> MAFVATQGATVVDQ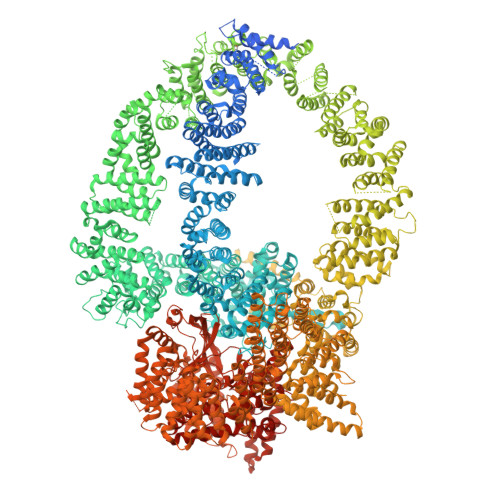TTLMKKYLQFVAALTDVNTPDETKLKMMQEVSENFENVTSSPQYSTFLEHIIPRFLTFLQDGEVQFLQEKPAQQLRKLVLEIIHRIPTNEHLRPHTKNVLSVMFRFLETENEENVLICLRIIIELHKQFRPPITQEIHHFLDFVKQIYKELPKVVNRYFENPQVIPENTVPPPEMVGMITTIAVKVNPEREDSETRTHSIIPRGSLSLKVLAELPIIVVLMYQLYKLNIHNVVAEFVPLIMNTIAIQVSAQARQHKLYNKELYADFIAAQIKTLSFLAYIIRIYQELVTKYSQQMVKGMLQLLSNCPAETAHLRKELLIAAKHILTTELRNQFIPCMDKLFDESILIGSGYTARETLRPLAYSTLADLVHHVRQHLPLSDLSLAVQLFAKNIDDESLPSSIQTMSCKLLLNLVDCIRSKSEQESGNGRDVLMRMLEVFVLKFHTIARYQLSAIFKKCKPQSELGAVEAALPGVPTAPAAPGPAPSPAPVPAPPPPPPPPPPATPVTPAPVPPFEKQGEKDKEDKQTFQVTDCRSLVKTLVCGVKTITWGITSCKAPGEAQFIPNKQLQPKETQIYIKLVKYAMQALDIYQVQIAGNGQTYIRVANCQTVRMKEEKEVLEHFAGVFTMMNPLTFKEIFQTTVPYMVERISKNYALQIVANSFLANPTTSALFATILVEYLLDRLPEMGSNVELSNLYLKLFKLVFGSVSLFAAENEQMLKPHLHKIVNSSMELAQTAKEPYNYFLLLRALFRSIGGGSHDLLYQEFLPLLPNLLQGLNMLQSGLHKQHMKDLFVELCLTVPVRLSSLLPYLPMLMDPLVSALNGSQTLVSQGLRTLELCVDNLQPDFLYDHIQPVRAELMQALWRTLRNPADSISHVAYRVLGKFGGSNRKMLKESQKLHYVVTEVQGPSITVEFSDCKASLQLPMEKAIETALDCLKSANTEPYYRRQAWEVIKCFLVAMMSLEDNKHALYQLLAHPNFTEKTIPNVIISHRYKAQDTPARKTFEQALTGAFMSAVIKDLRPSALPFVASLIRHYTMVAVAQQCGPFLLPCYQVGSQPSTAMFHSEENGSKGMDPLVLIDAIAICMAYEEKELCKIGEVALAVIFDVASIILGSKERACQLPLFSYIVERLCACCYEQAWYAKLGGVVSIKFLMERLPLTWVLQNQQTFLKALLFVMMDLTGEVSNGAVAMAKTTLEQLLMRCATPLKDEERAEEIVAAQEKSFHHVTHDLVREVTSPNSTVRKQAMHSLQVLAQVTGKSVTVIMEPHKEVLQDMVPPKKHLLRHQPANAQIGLMEGNTFCTTLQPRLFTMDLNVVEHKVFYTELLNLCEAEDSALTKLPCYKSLPSLVPLRIAALNALAACNYLPQSREKIIAALFKALNSTNSELQEAGEACMRKFLEGATIEVDQIHTHMRPLLMMLGDYRSLTLNVVNRLTSVTRLFPNSFNDKFCDQMMQHLRKWMEVVVITHKGGQRSDGNESISECGRCPLSPFCQFEEMKICSAIINLFHLIPAAPQTLVKPLLEVVMKTERAMLIEAGSPFREPLIKFLTRHPSQTVELFMMEATLNDPQWSRMFMSFLKHKDARPLRDVLAANPNRFITLLLPGGAQTAVRPGSPSTSTMRLDLQFQAIKIISIIVKNDDSWLASQHSLVSQLRRVWVSENFQERHRKENMAATNWKEPKLLAYCLLNYCKRNYGDIELLFQLLRAFTGRFLCNMTFLKEYMEEEIPKNYSIAQKRALFFRFVDFNDPNFGDELKAKVLQHILNPAFLYSFEKGEGEQLLGPPNPEGDNPESITSVFITKVLDPEKQADMLDSLRIYLLQYATLLVEHAPHHIHDNNKNRNSKLRRLMTFAWPCLLSKACVDPACKYSGHLLLAHIIAKFAIHKKIVLQVFHSLLKAHAMEARAIVRQAMAILTPAVPARMEDGHQMLTHWTRKIIVEEGHTVPQLVHILHLIVQHFKVYYPVRHHLVQHMVSAMQRLGFTPSVTIEQRRLAVDLSEVVIKWELQRIKDQQPDSDMDPNSSGEGVNSVSSSIKRGLSVDSAQEVKRFRTATGAISAVFGRSQSLPGADSLLAKPIDKQHTDTVVNFLIRVACQVNDNTNTAGSPGEVLSRRCVNLLKTALRPDMWPKSELKLQWFDKLLMTVEQPNQVNYGNICTGLEVLSFLLTVLQSPAILSSFKPLQRGIAACMTCGNTKVLRAVHSLLSRLMSIFPTEPSTSSVASKYEELECLYAAVGKVIYEGLTNYEKATNANPSQLFGTLMILKSACSNNPSYIDRLISVFMRSLQKMVREHLNPQAASGSTEATSGTSELVMLSLELVKTRLAVMSMEMRKNFIQAILTSLIEKSPDAKILRAVVKIVEEWVKNNSPMAANQTPTLREKSILLVKMMTYIEKRFPEDLELNAQFLDLVNYVYRDETLSGSELTAKLEPAFLSGLRCAQPLIRAKFFEVFDNSMKRRVYERLLYVTCSQNWEAMGNHFWIKQCIELLLAVCEKSTPIGTSCQGAMLPSITNVINLADSHDRAAFAMVTHVKQEPRERENSESKEEDVEIDIELAPGDQTSTPKTKELSEKDIGNQLHMLTNRHDKFLDTLREVKTGALLSAFVQLCHISTTLAEKTWVQLFPRLWKILSDRQQHALAGEISPFLCSGSHQVQRDCQPSALNCFVEAMSQCVPPIPIRPCVLKYLGKTHNLWFRSTLMLEHQAFEKGLSLQIKPKQTTEFYEQESITPPQQEILDSLAELYSLLQEEDMWAGLWQKRCKYSETATAIAYEQHGFFEQAQESYEKAMDKAKKEHERSNASPAIFPEYQLWEDHWIRCSKELNQWEALTEYGQSKGHINPYLVLECAWRVSNWTAMKEALVQVEVSCPKEMAWKVNMYRGYLAICHPEEQQLSFIERLVEMASSLAIREWRRLPHVVSHVHTPLLQAAQQIIELQEAAQINAGLQPTNLGRNNSLHDMKTVVKTWRNRLPIVSDDLSHWSSIFMWRQHHYQGKPTWSGMHSSSIVTAYENSSQHDPSSNNAMLGVHASASAIIQYGKIARKQGLVNVALDILSRIHTIPTVPIVDCFQKIRQQVKCYLQLAGVMGKNECMQGLEVIESTNLKYFTKEMTAEFYALKGMFLAQINKSEEANKAFSAAVQMHDVLVKAWAMWGDYLENIFVKERQLHLGVSAITCYLHACRHQNESKSRKYLAKVLWLLSFDDDKNTLADAVDKYCIGVPPIQWLAWIPQLLTCLVGSEGKLLLNLISQVGRVYPQAVYFPIRTLYLTLKIEQRERYKSDPGPIRATAPMWRCSRIMHMQRELHPTLLSSLEGIVDQMVWFRENWHEEVLRQLQQGLAKCYSVAFEKSGAVSDAKITPHTLNFVKKLVSTFGVGLENVSNVSTMFSSAASESLARRAQATAQDPVFQKLKGQFTTDFDFSVPGSMKLHNLISKLKKWIKILEAKTKQLPKFFLIEEKCRFLSNFSAQTAEVEIPGEFLMPKPTHYYIKIARFMPRVEIVQKHNTAARRLYIRGHNGKIYPYLVMNDACLTESRREERVLQLLRLLNPCLEKRKETTKRHLFFTVPRVVAVSPQMRLVEDNPSSLSLVEIYKQRCAKKGIEHDNPISRYYDRLATVQARGTQASHQVLRDILKEVQSNMVPRSMLKEWALHTFPNATDYWTFRKMFTIQLALIGFAEFVLHLNRLNPEMLQIAQDTGKLNVAYFRFDINDATGDLDANRPVPFRLTPNISEFLTTIGVSGPLTASMIAVARCFAQPNFKVDGILKTVLRDEIIAWHKKTQEDTSSPLSAAGQPENMDSQQLVSLVQKAVTAIMTRLHNLAQFEGGESKVNTLVAAANSLDNLCRMDPAWHPWL> GRQAGQQATVGRLRTQVTGFLSGALGKLQALSAQNMDPELAQFRVLDVDRAIMPLLIVAENARNPGLNLVPLHMDMAEDEEVRTQPPMA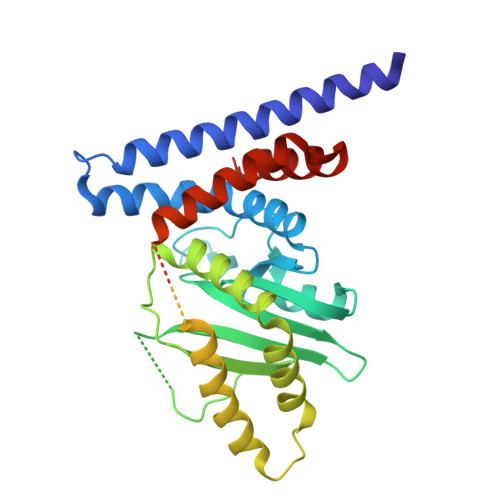GSRHIAEFVASARPGRYRAVIDDGSHTRAADIRKDASGTSVIVVDPLRKEKDESAYVDYADNVNMEFGEHAKCAFIPVDIQKSFFDCRILSLSLALKMHDKDDAFAAFHETLRNGGDPSHHVSRAQQTEELGATLVLDGAPLVDARMMKHGQAASSVSRYLGNHPEQSTVPVNKRNETLGERTTRHLVKRKVRNRADSEGRVTSGETKEITFSNSVEQKRIALLNRAASYVNSAPPPVVMRMAKLLQDSLLDTN>[2x]AYQLLLSKETLNKILQYKQNLEKGLATPGKFFLEELSKQEKSISEMDITTFTQLLIQSKKPQVFAESQVYHDGTDWTLEEESILGDVSVNMPVTMYNDGGHGSSFKNHPKPISGYLAYVPGALLASGSGPTSDMKEVLDNGKLNQDKLNALYERRLLPQLIHFNELARQNEKQAAITIPGIGTGCFSGAYYDVIKPYVRNALIHILEKHKDSLPYIDIIHYDPYMGDEPAEKKIGHMSF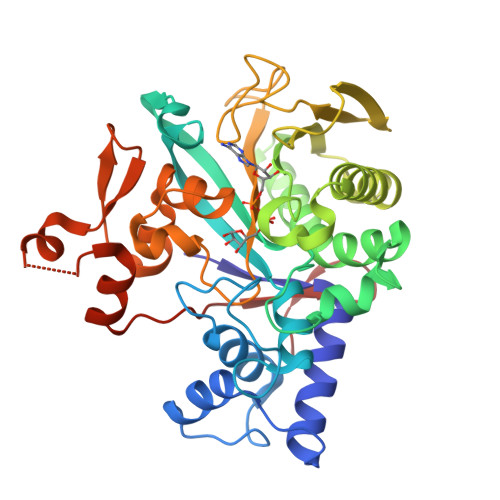RVSPSGVVRGTTGQLDYPLGSNPDTHILVSIVAWDHFSWPGNDYWGGARQTDDGVKAASTDTMGQVTGATGVYDKKWGRYMPPESFTKDRKGMSDWGDYVRENGIVFNGPVLALDKSGKLDTLE> QPSTANGGFPSVVVTAVTATTSISPDIESTWKGLLAGESGIHALEDEFVTKWDLAVKIGGHLKDPVDSHMGRLDMRRMSYVQRMGKLLGGQLWESAGSPEVDPDRFAVVVGTGLGGAERIVESYDLMNAGGPRKVSPLAVQMIMPNGAAAVIGLQLGARAGVMTPVSACSSGSEAIAHAWRQIVMGDADVAVCGGVEGPIEALPIAAFSMMRAMSTRNDEPERASRPFDKDRDGFVFGEAGALMLIETEEHAKARGAKPLARLLGAGITSDAFHMVAPAADGVRAGRAMTRSLELAGLSPADIDHVNAHGTATPIGDAAEANAIRVAGCDQA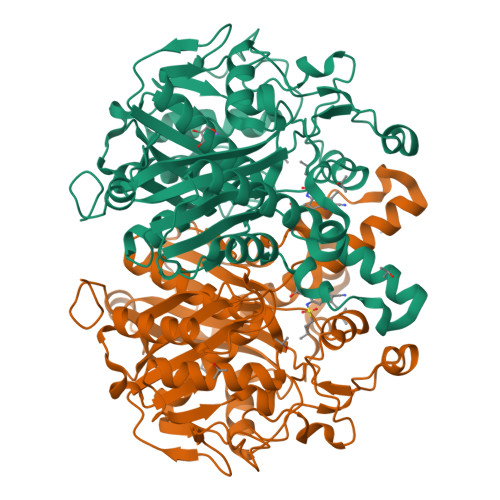AVYAPKSALGHSIGAVGALESVLTVLTLRDGVIPPTLNYETPDPEIDLDVVAGEPRYGDYRYAVNNSFGFGGHNVALAFGRY>LAFNEPLNVVSHLNDDWFLFGDSRSDCNHINNLSQQNYNYMDINPELCKSGKISAKAGNSLFKSFHFTDFYNYTGEGSQIIFYEGVNFTPYVGFKCLNNGDNNRWMGNKARFYTQLYQKMAHYRSLSVINITYTYNGSAGPVSMCKHIANGVTLTLNNPTFIGKEVSKPDYYYESEA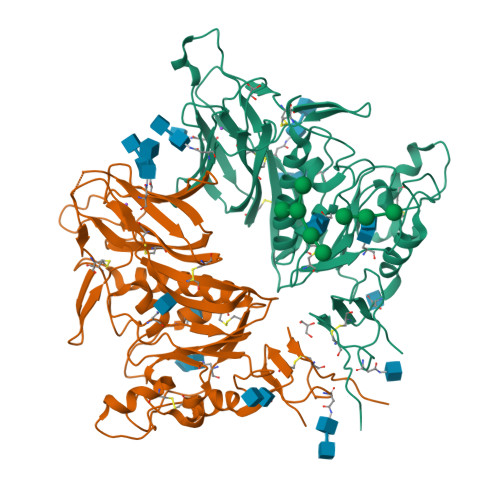NFTLQGCDEFIVPLCVFNGQYLSSKLYYDDSQYYYNVDTGVLYGFNSTLNITSGLDLTCIYLALTPGNYISISNELLLTVPSKAICLRKPKAFTPVQVVDSRWHSNRQSDNMTAIACQLPYCYFRNTTSDYNGVYDSHHGDAGFTSILAGLMYNVSCLAQQGAFVYNNVSSSWPQYPYGHCPTAANIVFMAPVCMYDSDPLVPR[2x]>[2x]AIKKTTEIDAILLNLNKAIDAHYQWLVSMFHSVVARDASK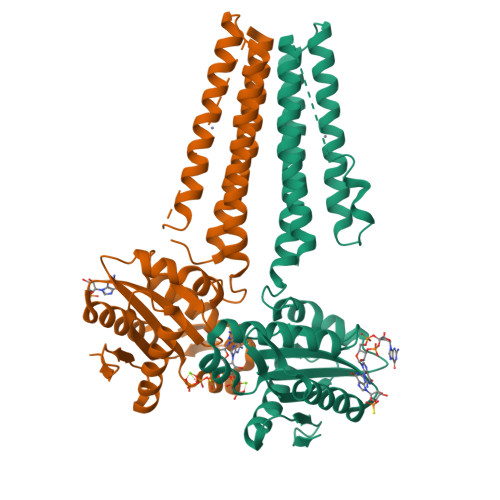PEITDNHSYGLAQFGRWIDHLGPLDNDELPYVRLMDSAHQHMHNCGRELMLAIVENHWQDAHFDAFQEGLLSFTAALTDYKIYLLTIRSNMDVLTGLPGRRVLDESFDHQLRNAEPLNLYLMLLDIDRFKLVNDTYGHLIGDVVLRTLATYLASWTRDYETVYRYGGEEFIIIVKAANDEEACRAGVRICQLVDNHAITHSEGHINITVTAGVSRAFPEEPLDVVIGRADRAMYEGKQTGRNRCMFIDEQNVINRVLEHHHHHH> G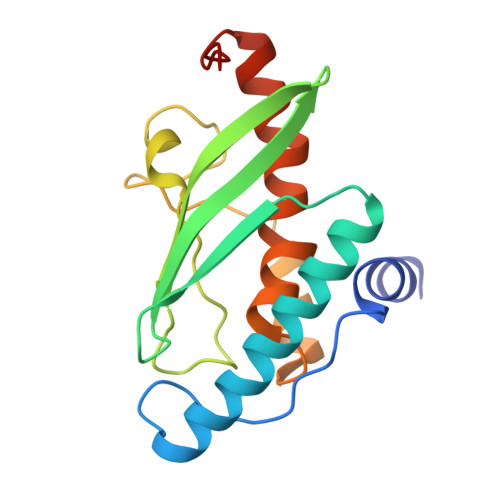SMADEATRRVVSEIPVLKTNAGPRDRELWVQRLKEEYQSLIRYVENNKNADNDWFRLESNKEGTRWFGKCWYIHDLLKYEFDIEFDIPITYPTTAPEIAVPELDGKAAKMYRGGKICLTDHFKPLWARNVPKFGLAHLMALGLGPWLAVEIPDLIQKGVIHHKEKCNQ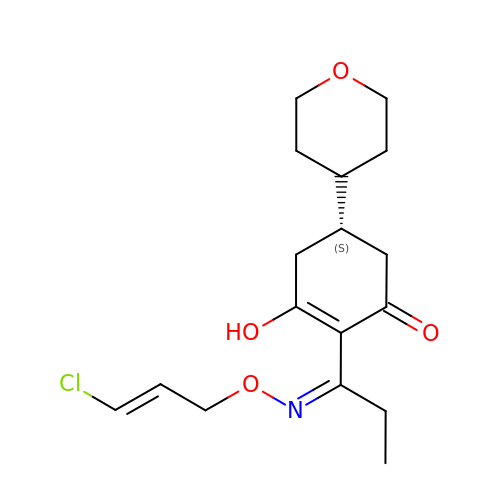(5S)-2-[(1E)-N-{[(2E)-3-chloroprop-2-en-1-yl]oxy}propanimidoyl]-3-hydroxy-5-(tetrahydro-2H-pyran-4-yl)cyclohex-2-en-1-one | C17 H24 Cl N O4 | IOYNQIMAUDJVEI-FGWLPLFYSA-N Human manganese superoxide dismutase (MnSOD) is a crucial oxidoreductase that maintains the vitality of mitochondria by converting superoxide (O2●−) to molecular oxygen (O2) and hydrogen peroxide (H2O2) with proton-coupled electron transfers (PCETs). Human MnSOD has evolved to be highly product inhibited to limit the formation of H2O2, a freely diffusible oxidant and signaling molecule. The Mn ion is bound by inner-sphere residues His26, His74, His163, Asp159, and a solvent molecule denoted as WAT1. The hydrogen bond network extends from WAT1 to outer-sphere residues Gln143, Tyr34, another solvent molecule denoted as WAT2, His30, and Tyr166 from the neighboring subunit.

Of particular interest is the Trp161Phe variant that decreases k2 by more than two orders of magnitude compared to wildtype, leading to exclusive use of the product-inhibited pathway as k2 « k3. The reduction of amino acid size at position 161 from tryptophan to phenylalanine leads to a slight lengthening of the distance between WAT1 and Gln143. From the cryocooled neutron structure of Trp161Phe Mn2+SOD, it is apparent that the Gln143-WAT1 hydrogen bonding interaction is perturbed compared to wildtype Mn2+SOD and may be the primary cause of the observed kinetic effects. The bulky Trp161 residue likely constrains Gln143 and WAT1 to form a SSHB for proton transfers. For the Trp161Phe reduced resting state, both chains have the same structure, and WAT1 is forming a hydrogen bond with the amide anion form of Gln143. For Trp161Phe Mn2+SOD, the protonation states of Tyr34, His30, and Tyr166 resemble those of the wildtype Mn2+SOD though there are notable structural features. Tyr34 engages in a 1.6 Å SSHB with WAT2 where Oη(Tyr34) acts as a hydrogen bond acceptor. Besides Tyr34, the other notable structural feature is the hydroxyl proton of Tyr166 that points away from His30. It is unclear whether the orientation of the proton has catalytic significance, is somehow related to the Trp161Phe variant, or is a consequence of cryocooling.

>[2x]MKHSLPDLPYDYGALEPHINAQIMQLHHSKHHAAYVNNLNVTEEKYQEALAKGDVTAQIALQPALKFNGGGHINHSIFWTNLSPNGGGEPKGELLEAIKRDFGSFDKFKEKLTAASVGVQGSGWGWLGFNKERGHLQIAACPNQDPLQGTTGLIPLLGIDVFEHAYYLQYKNVRPDYLKAIWNVINWENVTERYMACKK>MAKKTSSKGLKNPPGPWGWPLIGHMLTLGKNPHLALSRMSQQYGDVLQIRIGSTPVVVLSGLDTIRQALVRQGDDFKGRPDLYTFTLISNGQSMSFSPDSGPVWAARRRLAQNGLKSFSIASDPASSTSCYLEEHVSKEAEVLISTLQELMAGPGHFNPYRYVVVSVTNVICAICFGRRYDHNHQELLSLVNLNNNFGEVVGSGNPADFIPILRYLPNPSLNAFKDLNEKFYSFMQKMVKEHYKTFEKGHIRDITDSLIEHCQEKQLDENANVQLSDEKIINIVLDLFGAGFDTVTTAISWSLMYLVMNPRVQRKIQE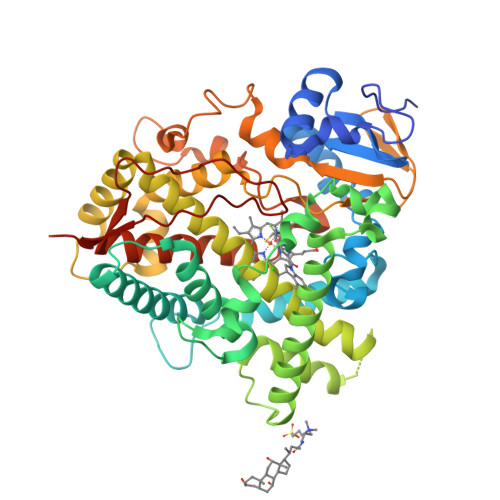ELDTVIGRSRRPRLSDRSHLPYMEAFILETFRHSSFVPFTIPHSTTRDTSLKGFYIPKGRCVFVNQWQINHDQKLWVNPSEFLPERFLTPDGAIDKVLSEKVIIFGMGKRKCIGETIARWEVFLFLAILLQRVEFSVPLGVKVDMTPIYGLTMKHACCEHFQMQLRSHHHHHH[4x]>[6x]MSISARNQLKGKVVGLKKGVVTAEVVLEIAGGNKITS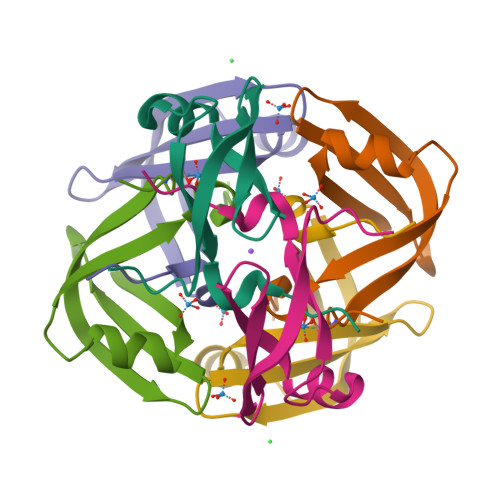IISLDSVEELGVKEGAELTAVVKSTDVMILA>[2x]MKLERLLSMKGGKGQDSYANNSLAQAMHARSMLHLLEETLENVHLNSSASPPPFTAVDLGCSSGANTVHIIDFIVKHISKRFDAAGIDPPEFTAFFSDLPSNDFNTLFQLLPPLVSNTCMEECLAADGNRSYFVAGVPGSFYRRLFPARTIDFFHSAFSLHWLSQVPESVT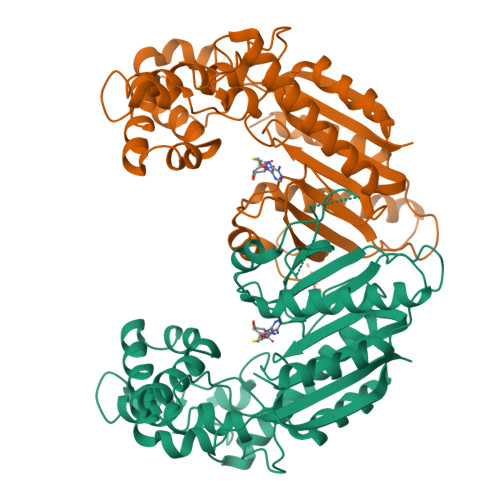DRRSAAYNRGRVFIHGAGEKTTTAYKRQFQADLAEFLRARAAEVKRGGAMFLVCLGRTSVDPTDQGGAGLLFGTHFQDAWDDLVREGLVAAEKRDGFNIPVYAPSLQDFKEVVDANGSFAIDKLVVYKGGSPLVVNEPDDASEVGRAFASSCRSVAGVLVEAHIGEELSNKLFSRVESRATSHAKDVLVNLQFFHIVASLSFT>QGNFTSKAAIHLTGGYNSESKTLDWRDDQDQAFSSGGLKLVNREIIIPDDGIYFVYSQVSLHISCTSELTEEQVL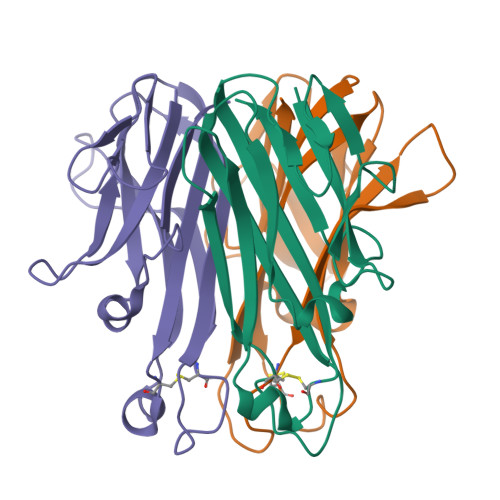MSHAVMRFSESYGGKKPLFSAIRSICTQEPESENLWYNTIYLGAAFHLREGDRLGTDTTTALLPMVENDNGKTFFGVFGL[3x]> LETFVGDQVLEIVPSNEEQIKNLLQLEAQEHLQLDFWKSPTTPGETAHVRVPFVNVQAVKVFLESQGIAYSIMIEDVQVLLDKENEEMLFNRRRERSGNFNFGAYHTLEEISQEMDNLVAEHPGLVSKVNIGSSFENRPMNVLKFSTGGDKPAIWLDAGIHAREWVTQATALWTANKIVSDYGKDPSITSILDALDIFLLPVTNPDGYVFSQTKNRMWRKTRSKVSGSLCVGVDPNRNWDAGFGGPGASSNPCSDSYHGPSANSEVEVKSIVDFIKSHGKVKAFIILHSYSQLLMFPYGYKCTKLDDFDELSEVAQKAAQSLRSLHGTKYKVGPICSVIYQASGGSIDWSYDYGIKYSFAFE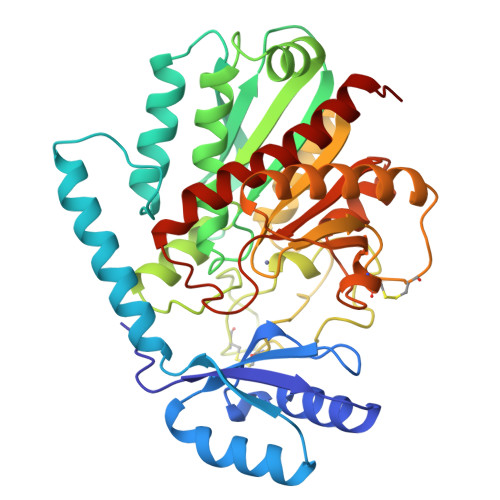LRDTGRYGFLLPARQILPTAEETWLGLKAIMEHVRDHPY>GNMSEVINFDQIFEGAIEPGKEPKRLFKEVYEGAITATSYAEILLSRAIEKYGPDHPVGYPDTAYFLPVIRAFSGEEVRTLKDMVPILNRMRAQIKSELTFENARLAGEATWYAAEIIEALRYLKHTPENPIVVPPWTGFIGDPVVRQYGIKMVDWTIPGEAIIIGRAKDSKAAKKIVDDLMGKGLMLFLCDEIIEQLLEENVKLGVDYIAYPLGNFTQVVHAANYALRAGLMFGGIAPGLRDAHRDYQRRRVLAFVLYLGEHDMVKTAAAMGAIFTGFPVITD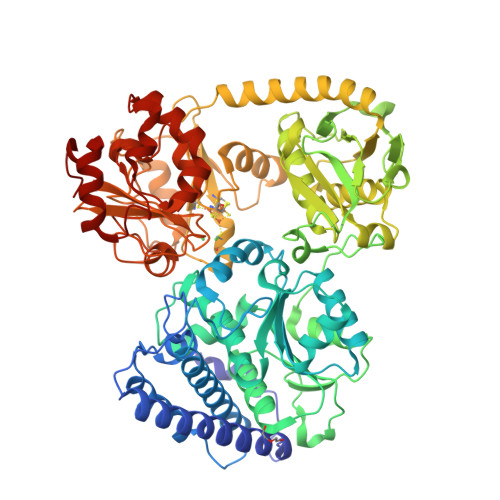QPLPEDKQIKDWFISEPDYDKIVQTALEVRGIKITSIDIDLPINFGPAFEGESIRKGDMHVEFGGGKTPSFELVRMVGPDEIEDGKVEVIGPDIDSVEPGGRLPIGIVVDIYGRKMQEDFEPVLERRIHYFTNYGEGFWHTAQRDLTWVRISKEAFAKGARLKHLGQLLYAKFKQEFPSIVDRVQVTIYTDEQKVLELREIARKKYAERDARLRELSDEAVDTYYSCLLCQSFAPTHVCIVSPERVGLCGAISWLDAKAAYEINPNGPNQPIPKEGLIDPVKGQWESFNEYIYKNSQRTIERMNLYTIMEYPMTSCGCFEAIMAYLPELNGFMIVNREHSGMTPIGMTFSTLAGMVGGGTQTPGFMGIGKSYIGSRKFVKADGGLARVVWMPKDLKEQLRSIIEERAEEEGLGRDFIDKIADETVGTTVDEVLPFLEEKGHPALSMEPLL[2x]>TALAEMPKRKFTIDDFDIVRPLGKGKFGNVYLAREKQNKFIMALKVLFKSQLEKEGVEHQLRREIEIQSHLRHPNILRMYNYFHDRKRIYLMLEFAPRGELYKELQKHGRFDEQRSATFMEELADALHYCHERKVIHRDIKPENLLMGYKGELKIADFGWSVHAPSLRRRTMCGTLDYLPPEMIEGKTHDEKVDLWCAGVLCYEFLVGMPPFDSPSHTETHRRIVNVDLKF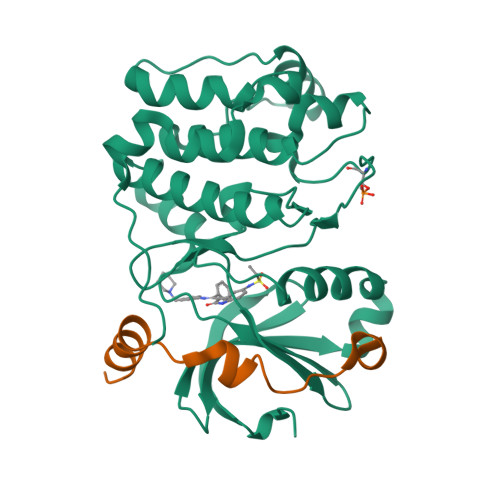PPFLSDGSKDLISKLLRYHPPQRLPLKGVMEHPWVKANSRRVLPPVYQSTQSK[2x];>[2x]IPAWASGNLLTQAIRQQYYKPIDVDRMYGTIDSPKLEELFNKS> AGTSCVNPPTVQNAYIVSRQMSKYPSGERVRYQCRSPYEMFGDEEVMCLNGNWTEPPQCKDSTGKCGPPPPIDNGDITSFPLSVYAPASSVEYQCQNLYQLEGNKRITCRNGQWS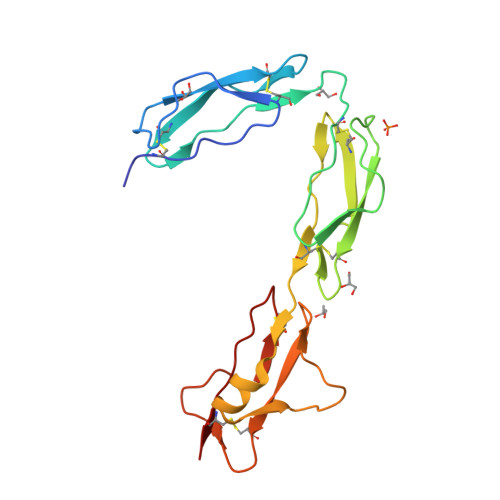EPPKCLHPCVISREIMENYNIALRWTAKQKLYSRTGESVEFVCKRGYRLSSRSHTLRTTCWDGKLEYPTCAKR>[6x]GSELTLRTIADEDDYESYMASAYSVFLRDPQKDEIEVNRKFTELDRMIGFHDGKKWVATTGAFSRHVVLPGGAVVPVAAVTAVTVSPTHRRRGLLTTMMRHQLADIRSRGESLAMLF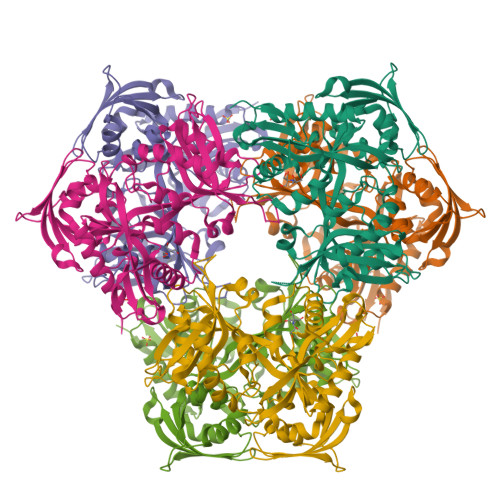ASEALIYGRFGYGVATESAELSGQVRELAFRPTVDLGDGTLEEVSAETFLASAPAIYDAVIPGLPGQMSRTPEWWASWTLDSEELQKESGKVRFVLHYESDGTASGFAIYRPKPGWGDAGPNAELHVQEVLGTNPRSYARTWRYLLDMDLVRKIKYHGASVQEELRYLVANHPSLECVVSDAIQVRLVDIPRALAQRRYAADVDVVLEVTDDFLPENSGRYRLRGGLDHASCEITTDDADIALTVRDLGSVYMGGVSLQVLASAGLVTELRAGAVQRAATAFGWPVAPSAPDDF> GSHMKIYIQPLSVN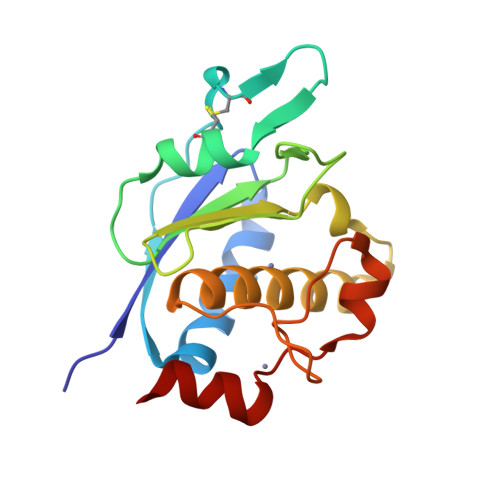SHTVEVLANSLPKIFNAEVFVLPASDVSLKCYNASRRQYNSTCILRMLPPIKVTLGVTGKDIYAKGMNFVFGEAELGGARAVLSVFRLTTADSELYRERVVKEAVHEIGHVLGLKHCSNNCVMRFSNSVQDVDRKPVSFCRECASKIRY> MEILRYLMDPDTFTSNFNNDPLVLRRRQTYLCYEVERLDNGTSVKMDQHMGFLCNESGRHAELRFLDLVPSLQLDPAQIYRVTWFISWSPCFSWGCAGEVRAFLQENTHVRLRIKAARIYDYDPLYKEALQMLRDAGAQVSIMTYDEFEYCWDTFVYRQGCPFQPWDG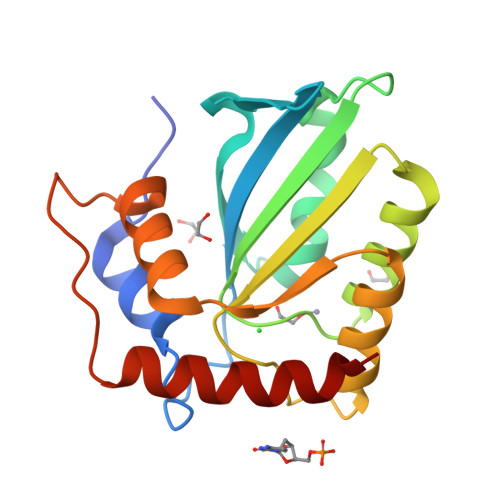LEEHSQALSGRLRAILQL Here, we report the crystal structure of the C-terminal hydrophilic domain of nsp4 (nsp4C) from MHV strain A59, together with the structure of a C425S site-directed mutant. The structure covers an 89 amino acid region from T408 to Q496 and is shown to possess a new fold. In particular, the C-terminal hydrophilic region from T408 to Q496 is highly conserved among all the coronaviruses, indicating that nsp4C may play a similar and conserved role in coronavirus replication.

The WT nsp4C monomer contains four α-helices (α1–α4) and two short β-strands (β1–β2). The refined WT model contains two nsp4C molecules in one asymmetric unit, termed A and B respectively. In the WT nsp4C structure, two monomers in one asymmetric unit are linked by a 2.0 Å Cys425-Cys425 disulfide bond to form a dimer. Notably, the N-termini of the two molecules are not aligned in the WT nsp4C dimer. Instead, they are projected in different orientations, with one molecule rotated by about 150° around the y-axis relative to the other molecule. The N-terminal amino acids Cys425, Lys421, Glu422, Lys426, and Asn429 are located in the contact surface between the two monomers. The hydrophobic cavity of WT nsp4C is exposed on the dimer surface, and the C-termini of the two monomers extend in different orientations. We propose that the surface properties of the WT nsp4C dimer are representative of an “open” conformation given that its positive, negative and hydrophobic areas are all exposed. In WT nsp4C, a disulfide bond at Cys425 causes the C-termini of the two monomers to extend in different orientations, and thus resulting in flexibility and undetectable electron density differences at the C-termini of the monomers. Our WT nsp4C crystal was obtained under non-reducing solutions, so it is considerably easier for two nsp4C monomers to form a disulfide bond in the crystal.

>[2x]GPLGSTFEEMALTTFMITKESYCKLKNSVSDVAFNRYLSLYNKYRYFSGKMDTAAYREAACSQLAKAMETFNHNNGNDVLYQPPTASVTTSFLQ> MGVALGATRVIYPAGQKQEQLAVTNNDENSTYLIQSWVENADGVKDGRFIVTPPL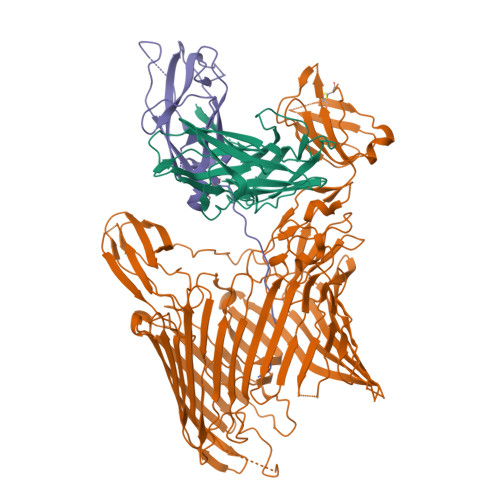FAMKGKKENTLRILDATNNQLPQDRESLFWMNVKAIPSMDKSKLTENTLQLAIISRIKLYYRPAKLALPPDQAAEKLRFRRSANSLTLINPTPYYLTVTELNAGTRVLENALVPPMGESTVKLPSDAGSNITYRTINDYGALTPKMTGVMEHHHHHH;> DLYFNPRFLADDPQAVADLSRFENGQELPPGTYRVDIYLNNGYMATRDVTFNTGDSEQGIVPCLTRAQLASMGLNTASVAGMNLLADDACVPLTTMVQDATAHLDVGQQRLNLTIPQAFMSNRARGYIPPELWDPGINAGLLNYNFSGNSVQNRIGGNSHYAYLNLQSGLNIGAWRLRDNTTWSYNSSDRSSGSKNKWQHINTWLERDIIPLRSRLTLGDGYTQGDIFDGINFRGAQLASDDNMLPDSQRGFAPVIHGIARGTAQVTIKQNGYDIYNSTVPPGPFTINDIYAAGNSGDLQVTIKEADGSTQIFTVPYSSVPLLQREGHTRYSITAGEYRSGNAQQEKPRFFQSTLLHGLPAGWTIYGGTQLADRYRAFNFGIGKNMGALGALSVDMTQANSTLPDDSQHDGQSVRFLYNKSLNESGTNIQLVGYRYSTSGYFNFADTTYSRMNGYNIETQDGVIQVKPKFTDYYNLAYNKRGKLQLTVTQQLGRTSTLYLSGSHQTYWGTSNVDEQFQAGLNTAFEDINWTLSYSLTKNAWQKGRDQMLALNVNIPFSHWLRSDSKSQWRHASASYSMSHDLNGRMTNLAGVYGTLLEDNNLSYSVQTGYAGGGDGNSGSTGYATLNYRGGYGNANIGYSHSDDIKQLYYGVSGGVLAHANGVTLGQPLNDTVVLVKAPGAKDAKVENQTGVRTDWRGYAVLPYATEYRENRVALDTNTLADNVDLDNAVANVVPTRGAIVRAEFKARVGIKLLMTLTHNNKPLPFGAMVTSESSQSSGIVADNGQVYLSGMPLAGKVQVKWGEEENAHCVANYQLPPESQQQLLTQLSAECRLVPRGSWSHPQFEK;> GNKWNTTLPGGNMQFQGVIIAETCRIEAGDKQMTVNMGQISSNRFHAVGEDSAPVPFVIHLRECSTVVSERVGVAFHGVADGKNPDVLSVGEGPGIATNIGVALFDDEGNLVPINRPPANWKRLYSGSTSLHFIAKYRATGRRVTGGIANAQAWFSLTYQ> MSDTMVVNGSGGVPAFLFSGSTLSSYRPNFEANSITIALPHYVDLPGRSNFKLMYIMGFPIDTEMEKDSEYSNKIRQESKISKTEGTVCYEQKITVETGQEKDGVKVYRVMVLEGTIAESIEHLDKKENEDILNNNRNRIVLADNTVINFDNISQLKEFLRRSVNIVDHDIFSSNGFEGFNPTSHFPSNPSSDYFNSTGVTFGSGVDLGQRSKQDLLNDGVPQYIADRLDGYYMLRGKEAYDKVRTAPLTLSDNEAHLLSNIYIDKFSHKIEGLFNDANIGLRFCDLPLRTRTALVSIGYQKGFKLSRTA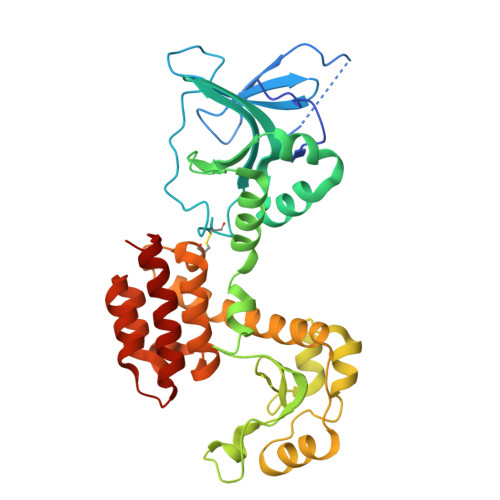PTVWNKVIAKDWNGLVNAFNNIVDGMSDRRKREGALVQKDIDSGLLK> NSVNPCCDPVICKPRDGEHCISGPCCNNCKFLNSGTICQRARGDGNHDYCTGIT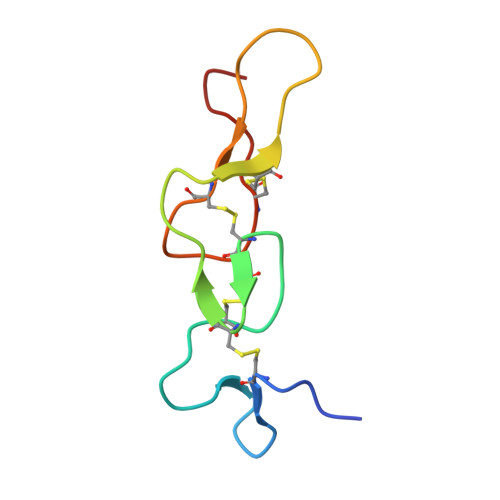TDCPRNRYNV phenyl N-[(1R)-3-oxidanylidene-1-phenyl-propyl]carbamate | C16 H15 N O3 | 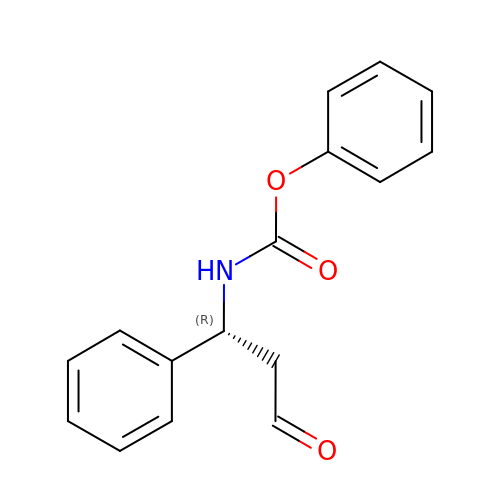HHWCOMIRIZKFCW-OAHLLOKOSA-N> MSAPPNTLFLRLEGALQSWGSNEAKFALRRTADAPTKSGVLGLLCAAMGIGRAEAADSWLPKLANLRMGVRIDRPGIRWWDFHTVGAGQRMRMAELKAPKKPSMVGAALAETLTPSKVKTRAETLLSRREYLADASFLVALQGEPELVAKLSAALAKPVWAIYLGRKSCPPSRPVCEHPPGFYNTLEEALSAVPLQKRWHNEPLPQILPCVMDWIPGYDGEHAPDDAEIHYDLPVSFQPPRHLPRFVIRRELVVGEDVQVSRETGTSVW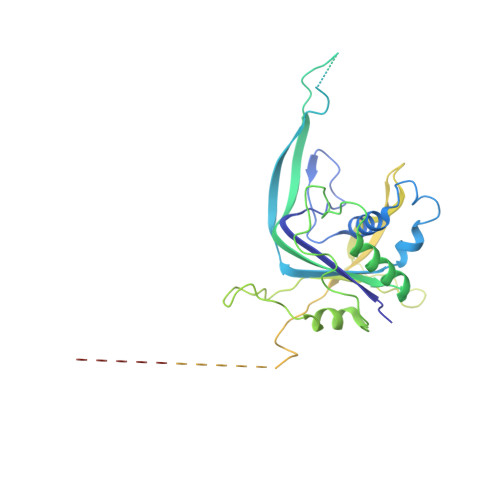RPKGTRADYNNSEYKKVRAERLVMDHAACMVCKHPATTVQHVNYRRAGGKEIPEDLRALCRLCHDACTMLEYGSGMTTNRIDPCDPIWRERILAKRKEIVEFRSRGQRFRKMKPEEENG> AKHLFTSESVSEGHPDKIADQISDAVLDAILEQDPKARVACETYVKTGMVLVGGEITTSAWVDIEEITRNTVREIGYVHSDMGFDANSCAVLSAIGKQSPDINQGVDRADPLEQGAGDQGLMFGYATNETDVLMPAPITYAHRLVQRQAEVRKNGTLPWLRPDAKSQVTFQYDDGKIVGIDAVVLSTQHSEEIDQKSLQEAVMEEIIKPILPAEWLTSATKFFINPTGRFVIGGPMGDCGLTGRK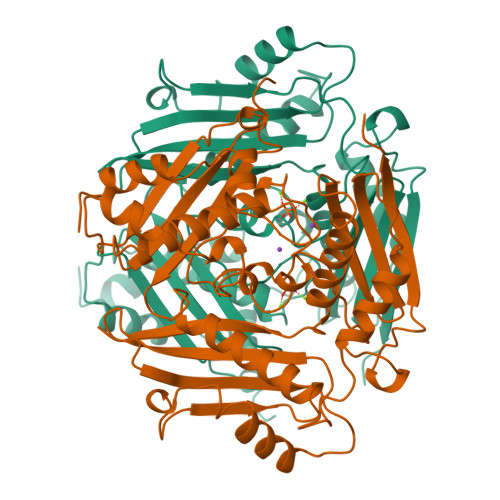IIVDTYGGMARHGGGAFSGKDPSKVDRSAAYAARYVAKNIVAAGLADRCEIQVSYAIGVAEPTSIMVETFGTEKVPSEQLTLLVREFFDLRPYGLIQMLDLLHPIYKETAAYGHFGREHFPWEKTDKAQLLRDAAGLK>[6x]MSKPQPIAAANWKCSGSPDSLSELIDLFNSTSINHDVQCVVASTFVHLAMTKERLSHPKFVIAA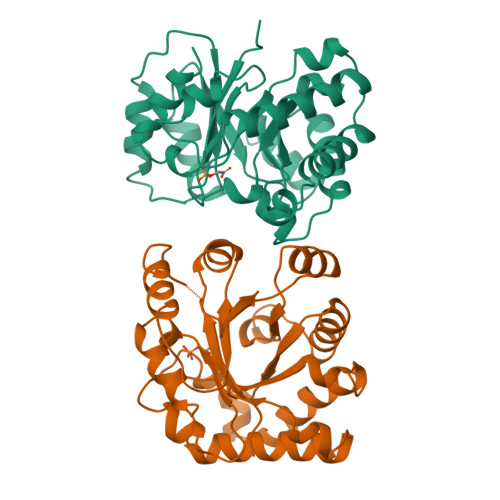QNAGNADALASLKDFGVNWIVLGHSERRWYYGETNEIVADKVAAAVASGFMVIACIGETLQERESGRTAVVVLTQIAAIAKKLKKADWAKVVIAYEPVWAIGTGKVATPQQAQEAHALIRSWVSSKIGADVAGELRILYGGSVNGKNARTLYQQRDVNGFLVGGASLKPEFVDIIKATQ>MAFKLPNLPYAYDALEPYIDQRTMEFHHDKHHNTYVTKLNATVEGTELEHQSLADMIANLDKVPEAMRMSVRNNGGGHFNHSLFWEILSPNSEEKGGVIDDIKAQWGTLDEFKNEFANKATTLFGSGWTWLVVNDGKLEIVTTPNQDNPLTEGKTPILLFDVWEHAYYLKYQNKRPDYMTAFWNIVNWKKVDELYQAA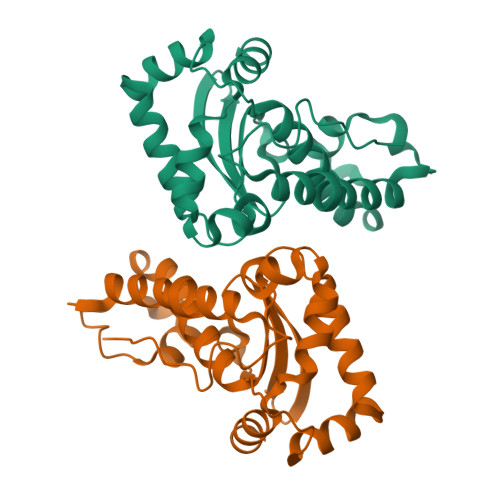K[2x]>GSHLTPELITSLQELSQILDRYDTIVFDLGDVLLHWDSVHFTSETKGIDDVRKMVKHPVWQDLEKGLINQEFALTALSCELETPCSKLKEMLELSIASLQVNPLMVEVLRVLHKKDKQIYCLSNVDLESFSYLYKQFDFWKYFDGIYVSALLQLRKPNPDIFQYLISSASINTKSTIFIDDKSENLQEAANFGISTLKYNKDNFEYTAIEGGWPIPLQNMTPEIHKKRTLGEDYLNLRLRKFPFCKSFVSNNVELIGGEDFSKEIFSTAVILHSYTSLPDDIIASMCHEILNHDGQNKLRWCFYKNEARPDNFPDDLNTTSMVLSFLLNHNKLTIEKIIPVAEQMIANRNEEGIIQVYFDDNRPRIDAIVAINVLYLMHQIGYGERKELKETEAFVFDFLISKEYLKGTRYYPAPDVFLFFLSRLVVDFPDQFEKFHKPLTEMLITRVNCSTFPLERALRIIALKKLGIVNRVDFLKLLDTQLADGGWPVYGLFIAPRSNTYFGSRELSTAFALEALHILS[2x]

In this study, we determined the co-crystal structures of drimenol synthase from Aquimarina spongiae (AsDMS), which catalyzes the conversion of farnesyl pyrophosphate (1) into drimenol (2). Crystallographic analyses of the enzyme bound to substrates 1 and drimenyl monophosphate (3) demonstrated that the TCβ domain catalyzes a class II cyclization reaction initiated by protonation, whereas the HAD domain catalyzes a phosphatase-like dephosphorylation reaction dependent on a divalent metal. Our results demonstrate that AsDMS is a bifunctional dimeric enzyme, comprising a protonation-initiated sesquiterpene cyclase (TCβ) domain and a metal-dependent HAD domain responsible for the stepwise release of phosphate to produce compound 2. The crystal structure revealed that AsDMS consists of N-terminal HAD and C-terminal TCβ domains connected by a highly flexible, disordered linker.

Additionally, to obtain a co-crystal structure with substrate 1, we introduced the D333N mutation into AsDMS d18 (AsDMS d18/D333N), which abolished the protonation-initiated cyclization reaction. To elucidate the cyclization mechanism catalyzed by the TCβ domain of AsDMS, we determined the crystal structure of substrate 1-bound AsDMS d18/D333N at a resolution of 2.60 Å. The electron density map of 1 was clearly observed at the center of the TCβ domain. Instead, it resembled merosterolic acid synthase, a monodomain class II cyclase that specifically recognizes the hydrophilic head of its substrate. Regarding the binding conformation of the pyrophosphate moiety, 1 formed salt bridges with the residues R378, R380, R425, and R513. 1 also formed hydrogen bonds with Y373 and Y426, and interacted with S514 through water-mediated hydrogen bonds. The hydrophobic tail of 1 adopts a binding conformation stabilized by interactions with multiple residues, grouped by their proposed functional roles: catalytic residues (D331, D333, and Y427), residues involved in π–cation interactions (F281, F318, F328, F509, and F518), and residues involved in van der Waals interactions (Y319, A511, and P512). The catalytic residue variants (D331A, D331N, D333N,30 and Y427F) exhibited a complete loss of enzymatic activity, supporting the idea that the D333 residue, which forms a hydrogen bond with the Y427 residue, catalyzes protonation at the C10 position of 1. The residue F518 was located near the C4 position of 1, suggesting that the C–H⋯π interaction between the carbocation intermediate and the aromatic ring of F518 determines the product selectivity.44 However, F518 is not appropriate for proton abstraction, and Y319 is clearly distant from the C4 carbocation. Initially, 1 binds within the TCβ domain, adopting an S-shaped conformation.>GSDELLYLPVRGRETYEMLLKIKESLELMQY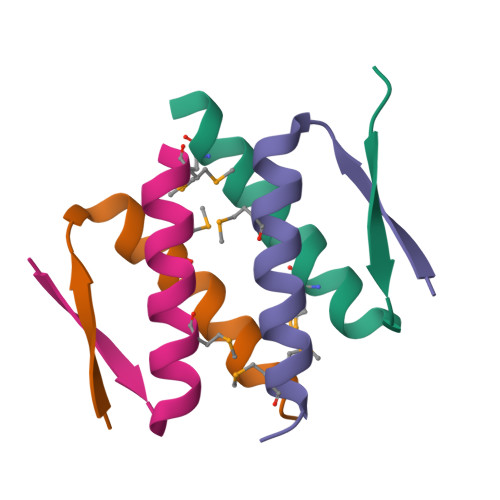L[4x]> HPETLVKVKDAEDQLGARVGYIELDLNSGKILESFRPEERFPLTSTFKVLLCGAVLSRVDAGQEQLGRRIHYSQNDLVEYSPVTEKHLTDGMTVRELCSAAITMSDNTAANLLLTTIGGPKELTDFLRQIGDKETRLDRIEPDLNEGKLGDLRDTTTPKAIASTLRKLLTGELLTLASRQQLIDWMEADKVAGPLLRSALPAGWFIADKSGAGERGSRGIIAALG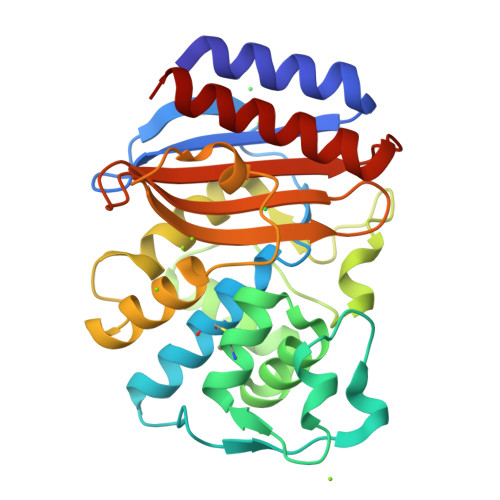PDGKPSRIVVIYTTGSQATMDERNRQIAEIGASLIKHW>GPLGSMPYSDAKAMLDEVAKIRELGVQRVTRIENLENAKKLWDNANSMLEKGNISGYLKAANELHKFMKEKNLKEDDLRPELSDKTISPKGYAILQSLWGAASDYSRAAATLTESTVEPGLVSAVNKMSAFFMDCKLSPNERATPDPDFKVGKSKILVGIMQFIKDVADPTSKIWMHNTKALMNHKIAAIQKLERSNNVNDETLESVLSSKGENLSEYLSYKYATKDEGREHRYTASTENFKNVKEKYQQMRGDALKTEILADFKDKLAEATDEQ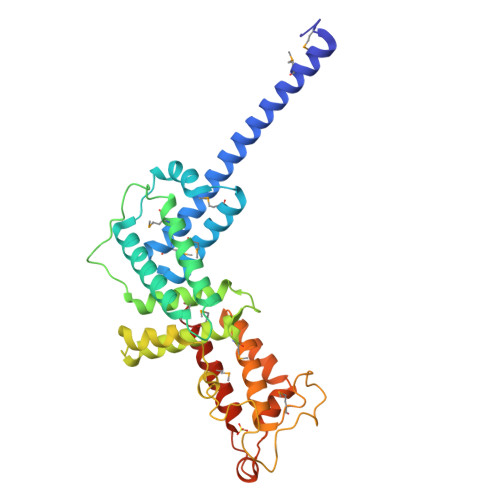SLKQIVAELKSKDEYRILAKGQGLTTQLLGLKTSSVSSFEKMVEETRESIKSQERQTIKIK[2x]>MNVDPHFDKFMESGIRHVYMLFENKSVESSEQFYSFMRTTYKNDPCSSDFECIERGAEMAQSYARIMNIKLETE[2x];>RFESVALEQLQIVHISSEADFSAVYSFRPKNLNYFVDIIAYEGKLPSTISEKSLGGYPVDKTMDEYTVHLNGR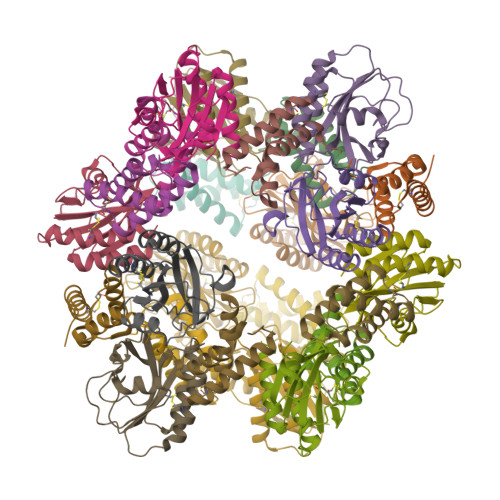HYYSNSKFAFLPTKKPTPEINYMYSCPYFNLDNIYAGTITMYWYRNDHISNDRLESICAQAARILGRAK[2x]The MUC2 mucin polymer is the main building unit of the intestinal mucus layers separating intestinal microbiota from the host epithelium. The MUC2 mucin is a large glycoprotein with a C-terminal domain similar to the MUC5AC and MUC5B mucins and the von Willebrand factor (VWF). The C-terminal part of MUC2 is made up by a VWD assembly, a series of VWC-domains and a C-terminal CK. A low-resolution image of the MUC2-C closely related MUC5B C-terminal has been published, but currently no high-resolution information is available for the mucins or VWF. Here, we present a model of the C-terminal part of MUC2 (MUC2-C) revealed by combining Cryo-EM and AlphaFold modeling which show an elongated dimer held together by covalent disulfide bonds in both ends.

To obtain further understanding, we expressed the MUC2-C in the presence of kifunensine to obtain N-glycans of the high-mannose type. Treatment with EndoH resulted in MUC2-C with only a single GlcNAc at the N-glycan sites. When this less glycosylated MUC2-C was analyzed by Cryo-EM (deglycosylated), it was only possible to resolve the VWC1 domain suggesting that the N-glycans restrain the flexibility of the MUC2-C tail. Alternatively, the less defined tail of the deglycosylated MUC2-C could be caused by its lower mass and increased difficulties in image analysis. The N-glycans were of di- to tetra-antennary type with a tendency for having the larger N-glycans found on the VWCN and VWD4 domains and the less complex ones on the MUC2-C tail.

>[2x]AAQPARRAVRSSRRHHHHHHGSGLEVLFQGPTPGTKPPECPDFDPPRQENETWWLCDCFMATCKYNNTVEIVKVECEPPPMPTCSNGLQPVRVEDPDGCCWHWECDCYCTGWGDPHYVTFDGLYYSYQGNCTYVLVEEISPSVDNFGVYIDNYHCDPNDKVSCPRTLIVRHETQEVLIKTVHMMPMQVQVQVNRQAVALPYKKYGLEVYQSGINYVVDIPELGVLVSYNGLSFSVRLPYHRFGNNTKGQCGTCTNTTSDDCILPSGEIVSNCEAAADQWLVNDPSKPHCPHSSSTTKRPAVTVPGGGKTTPHKDCTPSPLCQLIKDSLFAQCHALVPPQHYYDACVFDSCFMPGSSLECASLQAYAALCAQQNICLDWRNHTHGACLVECPSHREYQACGPAEEPTCKSSSSQQNNTVLVEGCFCPEGTMNYAPGFDVCVKTCGCVGPDNVPREFGEHFEFDCKNCVCLEGGSGIICQPKRCSQKPVTHCVEDGTYLATEVNPADTCCNITVCKCNTSLCKEKPSVCPLGFEVKSKMVPGRCCPFYWCESKGVCVHGNAEYQPGSPVYSSKCQDCVCTDKVDNNTLLNVIACTHVPCNTSCSPGFELMEAPGECCKKCEQTHCIIKRPDNQHVILKPGDFKSDPKNNCTFFSCVKIHNQLISSVSNITCPNFDASICIPGSITFMPNGCCKTCTPRNETRVPCSTVPVTTEVSYAGCTKTVLMNHCSGSCGTFVMYSAKAQALDHSCSCCKEEKTSQREVVLSCPNGGSLTHTYTHIESCQCQDTVCGLPTGTSRRARRSPRHLGSG> PSIKSGTILHAWNWSFNTLKHNMKDIHDAGYTAIQTSPINQVKEGNQGDKSMSNWYWLYQPTSYQIGNRYLGTEQEFKEMCAAAEEYGIKVIVDAVINHTTFDYAAISNEVKSIPNWTHGNTQIKNWSDRWDVTQNSLLGLYDWNTQNTQVQSYLKRFLERALNDGADGFRFDAAKHIELPDDGSYGSQFWPNITNTSAEFQYGEILQDSASRDAAYANYMDVTASNYGHSIRSALKNRNLGVSNISHYASDVSADKLVTWVESHDTYANDDEESTWMSDDDIRLGWAVIASRSGSTPLFFSRPEGGGNGVRFPGKSQIGDRGSALFEDQAITAVNRFHNVMAGQPEELSNPQGNNQIFMNQRGSHGVVL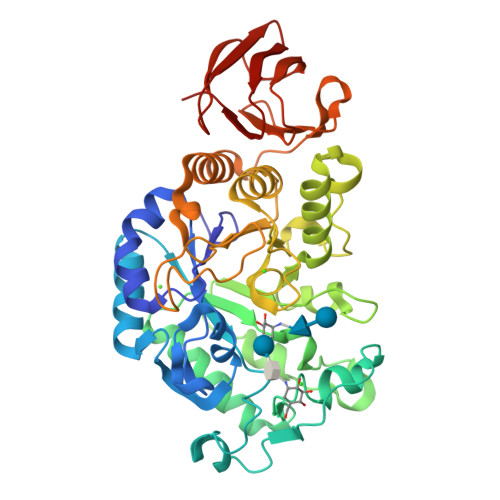ANAGSSSVSINTATKLPDGRYDNKAGAGSFQVNDGKLTGTINARSVAVLYPD>[2x]TQKPSLYRVLILNDDYTP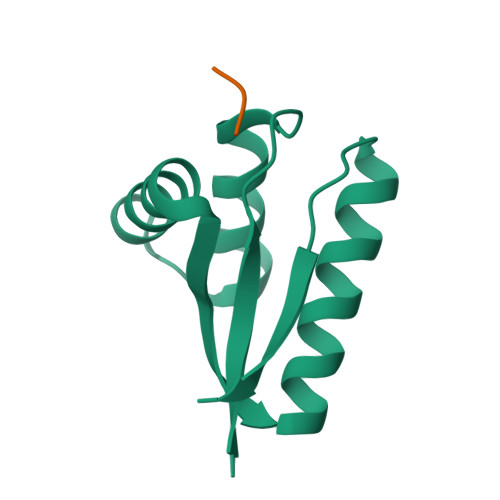MEFVVYVLERFFNKSREDATRIMLHVHQNGVGVCGVYTYEVAETKVAQVIDSARRHQHPLQCTMEKD;>YLFVQRDSKE[2x]>[24x]MGSSHHHHHHSSGLQGTENLYFQSHMSELIVNVINGPNLGRLGRREPAVYGGTTHDELVALIEREAAELGLKAVVRQSDSEAQLLDWIHQAADAAEPVILNAGGLTHTSVAL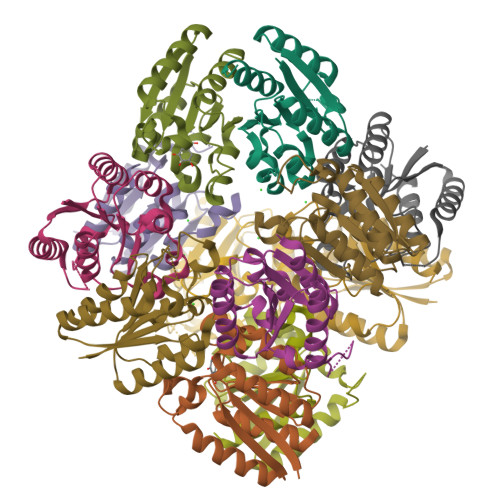RDACAELSAPLIEVHISNVHAREEFRRHSYLSPIATGVIVGLGIQGYLLALRYLAEHVGT> GSHMSKKILIVESDTALSATLRSALEGRGFTVDETTDGKGSVEQIRRDRPDLVVLAVDLSAGQNGYLICGKLKKDDDLKNVPIVIIGNPDGFAQHRKLKAHADEAVAKPVDADQLVERAGALIGFPE

The Myxococcus xanthus FrzS protein transits from pole-to-pole within the cell, accumulating at the pole that defines the direction of movement in social (S) motility. The N-terminal receiver domain (RD), a 258-residue coiled-coil domain, and the extreme C-terminal tail of the protein are all required for the dynamic subcellular localization and S-motility activity of FrzS. Here we show using atomic-resolution crystallography and NMR that the FrzS receiver domain (RD) displays the conserved switch Tyr102 in an unusual conformation, lacks the conserved Asp phosphorylation site, and fails to bind Mg2+ or the phosphoryl analogue, Mg2+·BeF3. The crystal structures of the mutants suggested that the observed conformation of Tyr102 in the wild-type FrzS RD is not sufficient for function. These results support the model that FrzS contains a novel ‘pseudo-receiver domain’ whose function requires recognition of the RD output face but not Asp phosphorylation.

We tested the functional importance of Tyr102 by mutating this residue to an alanine in FrzS-GFP and examining the social motility phenotype of the resulting strain. M. xanthus expressing FrzS-GFP Tyr102Ala failed to undergo normal colony expansion in the S-motility assay. Western blotting analysis showed equal levels of FrzS-GFP Tyr102Ala and wild-type FrzS-GFP in vivo, indicating that the phenotype of the Frz Tyr102Ala variant was not the result of decreased levels of the mutant protein. As these cells move forward over the agar surface, Tyr102Ala FrzS-GFP localizes primarily to the lagging cell pole in a manner highly reminiscent of FrzSΔRec-GFP. The Tyr102Ala mutant crystallized in similar conditions and in the same hexagonal space group as the high-resolution wild-type form. Similarly, no large rearrangements were seen in response to the loss of side-chain volume in the Tyr102Ala mutant. The overall Cα RMSD for the Tyr102Ala and wild-type RD structures was 0.23 Å. In response to this mutation, His92 switched to a more common rotamer that does not present Nδ1 to residue 102 for hydrogen bonding. There were no major structural rearrangements along the α4-β5-α5 face, and the all-atom RMSD for this area was low (0.43 Å). The close similarity of the Tyr102Ala and wild-type RD structures coupled with the loss of S-motility of the mutant suggests that the Tyr102 side chain plays a direct role in FrzS function.>SNAQIDGFVRTLRARPEAGGKVPVFVFHPAGGSTVVYEPLLGRLPADTPMYGFERVEGSIEERAQQYVPKLIEMQGDGPYVLVGWSLGGVLAYACAIGLRRLGKDVRFVGLIDAVRAGEEIPQTKEEIRKRWDRYAAFAEKTFNVTIPAIPYEQLEELDNEGQVRFVLDAVSQSGVQIPAGIIEHQRTSYLDNRAIDTAQIQPYDGHVTLYMADRYHDDAIMFEPRYAVRQPDGGWGEYVSDLEVVPIGGEHIQAIDEPIIAKVGEHMSR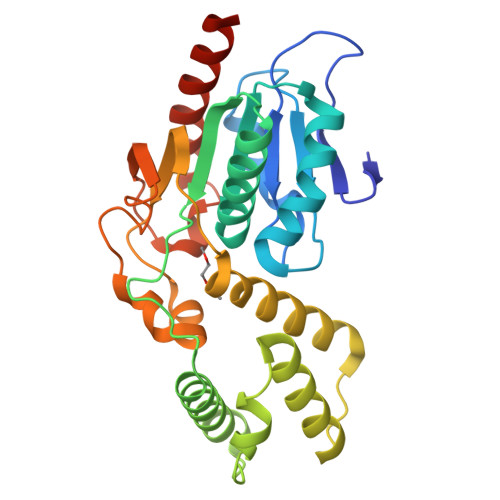ALGQIEADRTSEVGKQ[2x]> SEFGHRTLASTPALWASIPCPRSELRLDLVLPSGQSFRWREQSPAHWSGVLADQVWTLTQTEEQLHCTVYRGDKSQASRPTPDELEAVRKYFQLDVTLAQLYHHWGSVDSHFQEVAQKFQGVRLLRQDPIECLFSFICSSCNNIARITGMVERLCQAFGPRLIQLDDVTYHGFPSLQALAGPEVEAHLRKLGLGY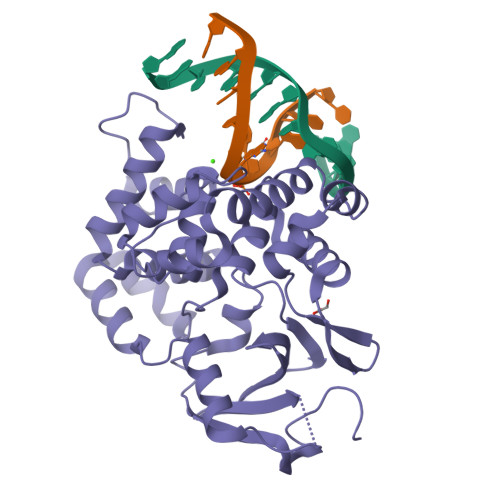RARYVSASARAILEEQGGLAWLQQLRESSYEEAHKALCILPGVGTKVADCICLMALDKPQAVPVDVHMWHIAQRDYSWHPTTSQAKGPSPQTNKELGNFFRSLWGPYAGWAQAVLFSADL> DHNDSIRASYMTIEELHDAGAALSRDGADSLPGFMEFDFFERHRENEKEILRVYRTTAVDAENGATITPAAEWLLDNHYVIEEAIQEVRRDFPRKFYRQLPTMTVGGVTIPRVMALGWLYVAHTHSTVSRENMTALVDGYQTSQTLQIGELWALPSIIRFVLIENLRRISIRVERSRRMRQKANEVVDEIIRLNDAEASAALLKQVDSLVDDPTFATQFLYRLRNGSQTSGFAVAWLEERLHAAGTDAENVMMSEHNRLASGNVTMGNIVKSLREIDDTEWSVWFEEVSHIDKVLREETDYEILDFGSRNTYRNTIELLARRSPRTEVE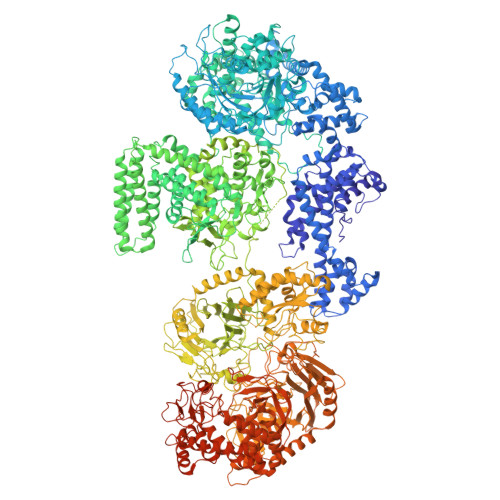VARAAVEMARSDLPAGADENHRVNVGSVLVGQRRFELEKALGYRPLASQHIVRSMRKFNWLAIAAPVLLITAVAMLAVGWFLAKAGMPWYVVTAFLLMFALPASEGATGLFNTLVTFFVKPFRLVGYEFKNGIPEDARTLVAVPCMLTSRDSVDEMMRNIEVHYLANPHGEIYFSLVSDWRDAPYEQSDEDLEILDYAKRELAALNSRYAFDGKTRFYLLHRRRIYNSAEECWMGWERKRGKLHELNMLLRGDKDTTFLGGSNIVPADVKYVMTLDADTRLMRDAVTKLVGKMHHPINRPKIDPVSGRVVEGYGLLQPRVTPSLTTGKDASVFQRVFSINRGIDPYVFTVSDVYQDLTSEGTFTGKGLYDVDAFEAALKGRIEENSILSHDLLEGSFARCALVTDVELVEDFPTRYEVEVSRQHRWARGDWQLLPFIIDRARGVTAIGRWKMVDNLRRSLTPIAWFFASILGWYFMDPLGALIWQILLIFSLFVAPTLSLLSGLVPRSTDIVPQAHFFTIWSEIRATNAQVALRIVFIADAACMMTDAIVRSLYRLLVSHKLMLEWRTAASMQSSAQGSIVDYYRQMWHAPVVAMLGLLFAALPGDNAFLIGIPFTLLWVLSPAVAWYVSQSAETEDRLFVSEHVSFELRKIARRTWRYYEAFVTPQENHLPPDNFQETPEPIVASRTSPTNIGVYLLSVISARQFGWISFADTLERIENTIQTVEKMEKHRGHLYNWYHTDTLQTLGPRYVSAVDSGNLAGHLIAVSSACRDWAEAPSAHLQGNLDGIGDVAGILRETLKALPDNRKTLRPLHRRLEERIIGFSNALASVKREHEFASIRVINLAVLARDIQKLATNVDHEVKSAQSAEVTRWAQLLVESCEAHISDSAIDLTNMEPLRQRLASLRDRSRNLAFSMDFTFLYRKDRRLLSIGYRVESKELDEACYDLLASECRLTSLFAIAKGDLPTEHWYRLGRQVVPIGAQGALVSWSGSMFEYLMPPLVMQERQGGILNQTNNLIVKEQMNHGRRLGTPWGISEAAFNARDHNMNYQYTNFGVPTLGLKRGLGQNAVIAPYASILASQYDPDGALENLDKLRKLGALGQYGFHDAVDFTPTRVPDGKVCAVVYNYYAHHHGMSIAAVANVAFDGVLRELFHSDPVIEAAELLLQEKAPREVPVMSAKYEPETPGKEQADLLRAEVRSIADPAVRDREVVFLSNGHYSTMLTSTGAGYSKWNGQAISRWKADPTDDRWGTFIFLRDTTNGQWWSATAEPRVIEGEKTKTIFTDDKAEFHKTIGDLQSVVECIVATEHDAEGRRITLLNVGSEDRYIEVTSYMEPVIASEDDDNAHPLFSRMFVQTEIGRRGDVIRAWRNRRSQNEPGTVIAHLAADNAGPSRPTEFETDRAKFIGRGRSLREAAAFDAGATLSSSDGFTLDPILSLRRTVRVPAGKKVSVIFWTIAAPSREEVDKAIDRYRHPDAFAHELVHAWTRTQVQMRHVGVTSQQAAAFQHLGRYLTYPDMHLRADSETLKTGLASQRALWPLAISGDFPIFSLRINDDMDMDIAREALSAHEYLRSRGVIFDLVIVNERAASYAQDMQHALDHISETQRRINPADGGRPHVFSVRRDLMDEETWSALLAASRVVLHVRNGKIVDQINRAVSLFAANRGPDGSSDAAQARLPVPAFPVAEPVEDAGDLDFWNGFGGFAKNGQEYVVRLNGGQSTPHPWINVISNENFGFHISAEGAGFSWSRNSRDYQLTPWTNDPVINRPGEAFYVADVETGKLYTPCAALSRDPEAMFETRHGLGYSILTGVADTLEVELTQTVDREKPVKFSQVIVRNKGSKSRRLKVYAYVEWVLGNNGQKSAPFILSRHDAGSNAIFASNPYSIDYSARTSFLTLDSEASGFTTSRREFIGRFGSAQAPQGIVAGAALSGTTEVDGDPCAALMQEIHLKPGEERHMTFILGDADNAEEAEALVKDVRQADFLSVLEESKKFWTGFTGQLQVSTPDAGFNHMVNNWLPYQALACRILARTAFYQSSGAFGFRDQLQDTLAFLLYQPDLARTQILRAAGRQFPEGDVQHWWLPLTGAGVRTTISDDVVWLAYAINQYVSATGDAAILDESIPFLKGPALMPGQHDAFFQPETSERSATLYEHAALALDLAIHRTGENGLPLILGGDWNDGMNRVGVGGKGTSVWLGWFLAGALRDFIEIAEKRGDTDRVGKWASHREKLRHVLETAGWDGSYYRRGYFDDGTPLGSASSEECQIDSLGQSWSVLSGEGEEGRSRQAMDAVMEHLVDEKTGIIRLFTPPFSRASHDPGYIKGYPPGVRENGGQYTHAATWVVLALAKQGRAQEAWNCFKLLNPVNHALDAASSETYRVEPYVVTADVYGEGAYAGRGGWSWYTGSAGWLYRAAVEGILGITRTDGKLHVSPSLPEDWSGFSIRITLDGKARDIAVSRKAGTADVSVSVDG>MSTGPDFIYDDRPAAVSSTFNPEKGYMDFITAYGKNINADNVRIFFLNHKKAKDSLKGSPKVEVDLQFGTLRVKVVNNHNPRNRDNPVADNAITLHRLSGYLAKWCFDEIDHGQIEEAEVKSKVVIPLAEAKGCKWGDGVAL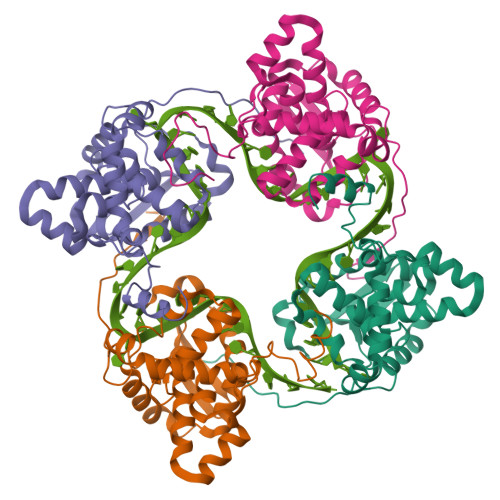YLAFAPGAEMFLKDFEFYPLAIDIQRVVKDGMDITFMRKVLKQRYGTKTADDWMISEVTAIQSAVKVVAKLPWAKAGFTAAAKNFLAKFNISV[4x]>MREYKLVVLGSGGVGKSALTVQFVQGIFVDEYDPTIEDSYRKQVEVDAQQCMLEILDTAGTEQFTAMRDLYMKNGQGFALVYSITAQSTFNDLQDLREQILRVKDTDDVPMILVGNKCDLEDERVVGKEQGQNLARQWNNCAFLESSAKSKINVNEIFYDLVRQINR[2x];>M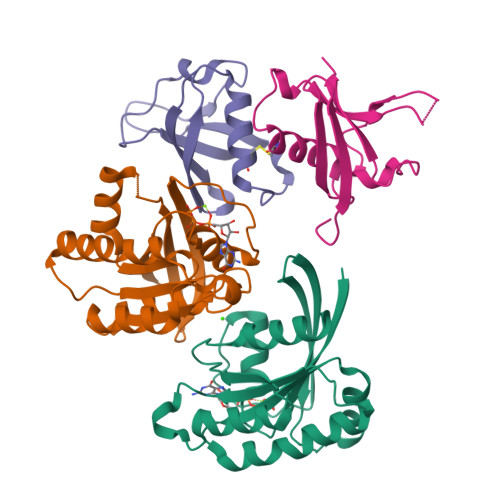DGPGASAVVVRVGIPDLQQTKCLRLDPAAPVWAAKQRVLCALNHSLQDALNYGLFQPPSRGRAGKFLDEERLLQEYPPNLDTPLPYLEFRYKRRVYAQ[2x]>[6x]GSASNPQTEEVSIKEIAITHHVKEGHEKADPSQFELLKVLGQGSFGKVFLVKKISGSDARQLYAMKVLKKATLKVRDRVRTKMERDILVEVNHPFIVKLHYAFQTEGKLYLILDFLRGGDLFTRLSKEVMFTEEDVKFYLAELALALDHLHSLGIIYRDLKPENILLDEEGHIKLTDFGLSKESIDHEKKAYSFCGTVEYMAPEVVNRRGHTQSADWWSFGVLMFEMLTGTLPFQGKDRKETMTMILKAKLGMPQFLSPEAQSLLRMLFKRNPANRLGAGPDGVEEIKRHSFFSTIDWNKLYRREIHPPFKPATGRP;>GSRMLPIEGAPRRRPPVKFIFPPPPLSSLPGFGRPRGYAGPTVIDMSAPDDVFAEDTPSPPAT[6x]

The Kaposi’s sarcoma associated herpesvirus protein ORF45 binds the extracellular signal-regulated kinase (ERK) and the p90 Ribosomal S6 kinase (RSK). ERK and RSK are key downstream components of the epidermal growth factor (EGF)/Ras/ERK pathway. RSK consists of two kinase domains connected by a flexible linker. To understand how ORF45 forms a complex with both ERK and RSK and causes persistent activation of the two kinases, we determined the crystal structures of ppERK2-ORF45 and RSK(NTK)-ORF45 binary complexes.

To reveal the structural basis of NTK-ORF45 binding, we determined the crystal structure of the NTK-ORF45(16-76) complex at 2.75 Å resolution. The asymmetric unit contained 6 NTK-ORF45 complexes and 47 amino acids from ORF45 could be traced in the electron density map. ORF45 makes contacts with the C-lobe of the NTK. The NTK/VF-motif crystal structure showed how the valine and phenylalanine side-chains snugly fit into a small hydrophobic pocket and highlighted the importance of other neighboring D/E residues involved in electrostatic interactions. As expected, binding affinity decreased by ~100-1000-fold when F268 was changed to serine or L285, M287 or R305 were replaced with alanine or with bulkier tryptophan/phenylalanine residues. The NTK(WT)-ORF45 interaction has a slow on-rate because of the structural rearrangement that needs to take place before VF-motif binding since L285 is incompatible with F66(ORF45) in its original position. The VF-motif binding groove by the αG/αH region at the bottom of the NTK C-lobe, to our knowledge, has so far not been reported as a linear motif binding surface.>[2x]MAHHHHHHVDDDDKMADVTAQAVATW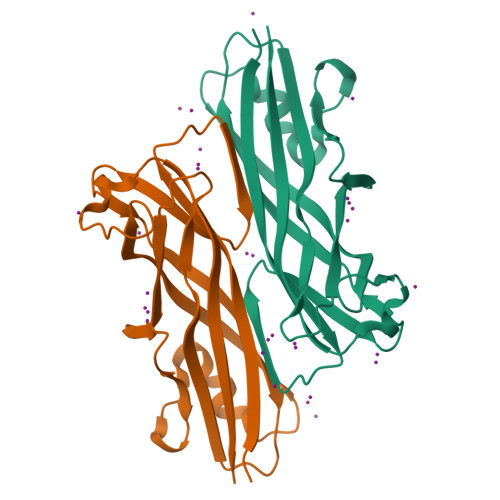SATAKKDTTSKLVVTPLGSLAFQYAEGIKGFNSQKGLFDVAIEGDSTATAFKLTSRLITNTLTQLDTSGSTLNVGVDYNGTAVEKTGDTVMIDTANGVLGGNLSPLANGYNASNRTTAQDGFTFSIISGTTNGTTAVTDYSTLPEGIWSGDVSVQFDATWTS>RIMKLDDERQTETYITQINPEGKEMYFASGLGNLYT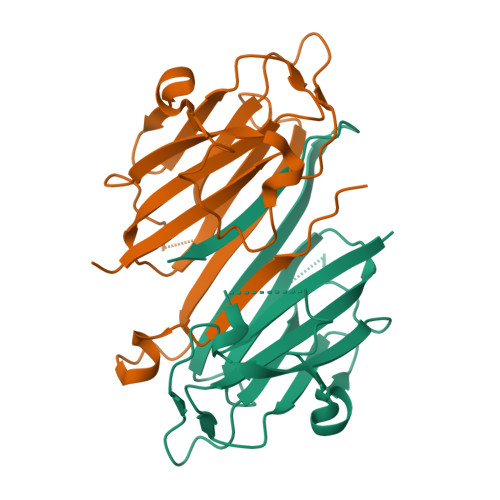IIGSDGTSGSPVNLLNAEVKILKTNSKNLTDSMDQNYDSPEFEDVTSQYSYTNDGSKITIDWKTNSISSTTSYVVLVKIPKQSGVLYSTVSDINQTYGSKYSYGHTNISGDSDANAEIKLLSLEHHHHHH[2x]>[12x]MKYVVVSGGVISGIGKGVLASSTGMLMKTLGLKVTSIKIDPYMNIDAGTMSPLEHGECFVLDDGGETDLDLGNYERYLGVTLTKDHNITTGKIYSHVIAKERKGDYLGKTVQIVPHLTNAIQDWIERVAKIPVDDTGMEPDVCIIELGGTVGDIESAPFVEALRQFQFKVGKENFALIHVSLVPVIHGEQKTKPTQAAIKGLRSLGLVPDMIACRCSETLDKPTIDKIAMFCHVGPEQVVNVHDVNSTYHVPLLLLEQKMIDYLHA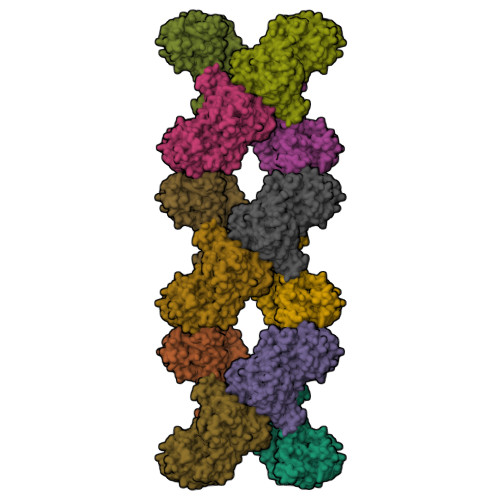RLKLDEISLTEEEKQRGLELLSKWKATTGNFDESMETVKIALVGKYTNLKDSYLSVIKALEHSSMKCRRKLDIKWVEATDLEPEAQESNKTKFHEAWNMVSTADGILIPGGFGVRGTEGMVLAARWARENHIPFLGVCLGLQIATIEFTRSVLGRKDSHSAEFYPDIDEKNHVVVFMMRLGLRPTFFQNETEWSQIKKLYGDVSEVHERHRHRYEINPKMVDELENNGLIFVGKDDTGKRCEILELKNHPYYIATQYHPEYTSKVLDPSKPFLGLVAASAGILQDVIEGKYDLEA CRM197 is a genetically detoxified mutant of diphtheria toxin (DT) that is widely used as a carrier protein in conjugate vaccines. CRM197 is the G52E mutant of DT, which renders it catalytically inactive and thus nontoxic, without the lysine adducts and heterogeneity that result from formaldehyde treatment. Wild-type DT has been described in two oligomeric forms: a monomer and a domain-swapped dimer. The hinge connects the large module comprising the N-terminal (catalytic and transmembrane) domains to the C-terminal (receptor-binding) domain.

Here, CRM197 was expressed as a soluble, intracellular protein in an Escherichia coli strain engineered to have an oxidative cytoplasm. The purified product, called EcoCRM, remained monomeric throughout crystallization. The structure of monomeric EcoCRM is reported at 2.0 Å resolution with the domain-swapping hinge loop (residues 379–387) in an extended, exposed conformation, similar to monomeric wild-type DT. Three internal zones are missing due to disorder. The first zone is residues 30–33, a surface loop near the active site, and the second is residues 39–49, which form the active-site loop that is only fully ordered in wild-type structures that include a substrate analog. The G52E mutation site is well ordered in the present structure. The third disordered zone comprises residues 187–200. Based on comparing the pH across known structures (including during protein preparation), it is likely that maintaining a high pH and avoiding phosphate were important in maintaining the monomeric state observed in the present report. The dimer conformation gains two positive-φ residues, Gly383 and Lys385, and is more compact; the Cα distance between Tyr380 and Pro388 decreases from 16.0 to 9.8 Å. In CRM197, the side chain of Lys385 in the hinge loop is more solvent-exposed in the monomeric structure (SASA of 91.6 Å2) than in the dimer (SASA of 2.4 Å2).

> GADDVVDSSKSFVMENFSSYHGTKPGYVDSIQKGIQKPKSGTQGNYDDDWKEFYSTDNKYDAAGYSVDNENPLSGKAGGVVKVTYPGLTKVLALKVDNAETIKKELGLSLTEPLMEQVGTEEFIKRFGDGASRVVLSLPFAEGSSSVEYINNWEQAKALSVELEINFETRGKRGQDAMYEYMAQACAGNRVRRSVGSSLSCINLDWDVIRDKTKTKIESLKEHGPIKNKMSESPNKTVSEEKAKQYLEEFHQTALEHPELSELKTVTGTNPVFAGANYAAWAVNVAQVIDSETADNLEKTTAALSILPGIGSVMGIADGAVHHNTEEIVAQSIALSSLMVAQAIPLVGELVDIGFAAYNFVESIINLFQVVHNSYNRPAYSPGHKTQPFLHDGYAVSWNTVEDSIIRTGFQGESGHDIKITAENTPLPIAGVLLPTIPGKLDVNKSKTHISVNGRKIRMRCRAIDGDVTFCRPKSPVYVGNGVHANLHVAFHRSSSEKIHSNEISSDSIGVLGYQKTVDHTKVNSKLSLFFEIKS> SAGXA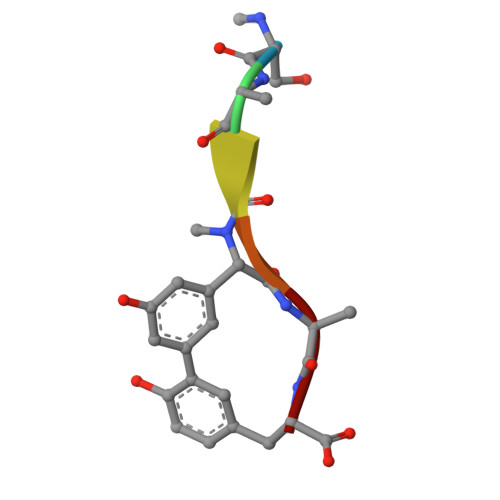Y>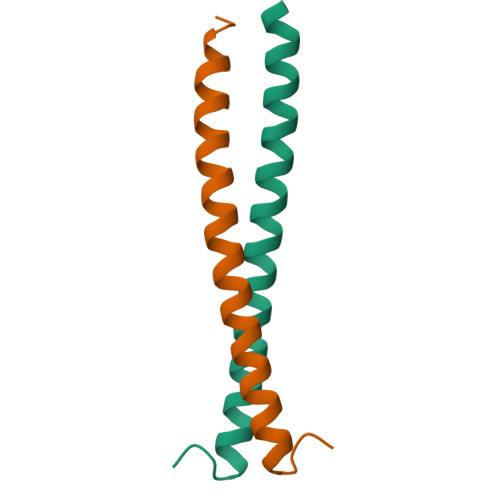[4x]GSERQILRLKQINIQLATKIQHLEFSCSEKEQEIERLNKLLKQNGLLGDVN[(2S)-3-[(2S)-2-(disulfanyl)-2,3-dihydro-1H-imidazol-4-yl]-1-oxidanyl-1-oxidanylidene-propan-2-yl]-trimethyl-azanium | C9 H18 N3 O2 S2 | 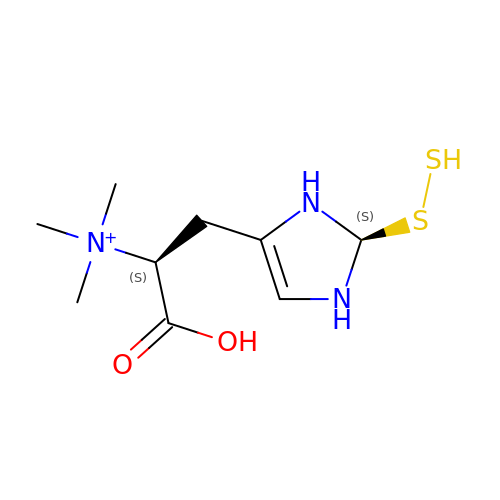XGMLHKDWXWTLLL-CBAPKCEASA-O> MEPGPTAAQRRCSLPPWLPLGLLLWSGLALGALPFGSSPHRVFHDLLSEQQLLEVEDLSLSLLQGGGLGPLSLPPDLPDLDPECRELLLDFANSSAELTGCLVRSARPVRLCQTCYPLFQQVVSKMDNISRAAGNTSESQSCARSLLMADRMQIVVILSEFFNTTWQEANCANCLTNNSEELSNSTVYFLNLFNH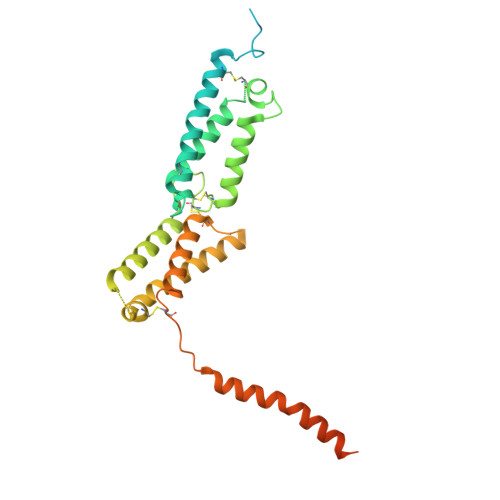TLTCFEHNLQGNAHSLLQTKNYSEVCKNCREAYKTLSSLYSEMQKMNELENKAEPGTHLCIDVEDAMNITRKLWSRTFNCSVPCSDTVPVIAVSVFILFLPVVFYLSSFLHSEQKKRKLILPKRLKSSTSFANIQENSNLEHHHHHHHH> MHSTLRVFTKNNCLSFTNMNRFSTAAQVAQANYSKFRADYSASVAAFQQRIKTIEKENTGSMKKPMAKAYEHPYNSEHHPLNFSAVKIAETFHDFIGPEQVSPHYESFAMSRKFLLTFWGGFFVLNFGMATVDLNWIMKSTYIPWIFWFQLMYFYVEGKNSMFMPLLQRFYRRAAANEIFTMEAFYHENIENKLRNLMRITKGQLEYWDIHTSYGEIRADSINNFLANEYLRLQSHITSRALNILKQAQAYETMNQAALLQKL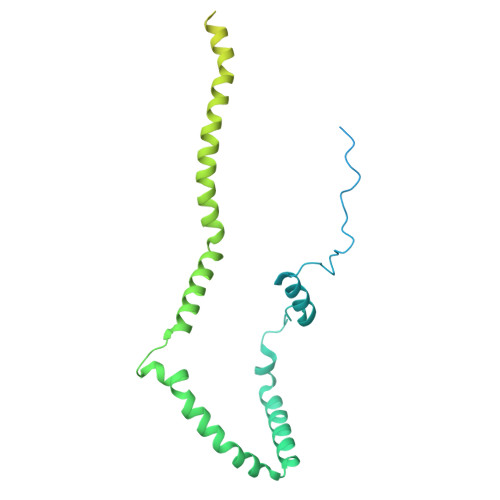IDDATSAIDNALKGDKKAEVLARSLDSAIDGLSKGYMDYQNDPLLPLILSSIEANVKKITTLSAQEQANLIGLTAEQLKSIKENDVRARKEFLESQPKLDNNLKNIESVKKILATWGK> MVDGNYSVASNVMVPMRDGVRLAVDLYRPDADGPVPVLLVRNPYDKFDVFAWSTQSTNWLEFVRDGYAVVIQDTRGLFASEGEFVPHVDDEADAEDTLSWILEQAWCDGNVGMFGVSYLGVTQWQAAVSGVGGLKAIAPSMASADLYRAPWYGPGGALSVEALLGWSALIGRGLITSRSDARPEDAADFVQLAAILNDVAGAASVTPLAEQPLLGRLIPWVIDQVVDHPDNDESWQSISLFERLGGLATPALITAGWYDGFVGESLRTFVAVKDNADARLVVGPWSHSNLTGRNADRKFGIAATYPIQEATTMHKAFFDRHLRGETDALAGVPKVRLFVMGIDEWRDETDWPLPDTAYTPFYLGGSGAANTSTGGGTLSTSISGTESADTYLYDPADPVPSLGGTLLFHNGDNGPADQRPIHDRDDVLCYSTEVLTDPVEVTGTVSARLFVSSSAVDTD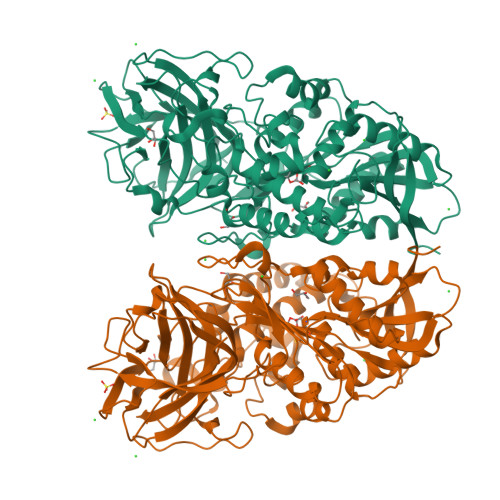FTAKLVDVFPDGRAIALCDGIVRMRYRETLVNPTLIEAGEIYEVAIDMLATSNVFLPGHRIMVQVSSSNFPKYDRNSNTGGVIAREQLEEMCTAVNRIHRGPEHPSHIVLPIIKRKLAAALEHHHHHH3-[1-[3-[(4~{S})-6-azanyl-5-cyano-3-methyl-4-propan-2-yl-2~{H}-pyrano[2,3-c]pyrazol-4-yl]-5-(trifluoromethyl)phenyl]piperidin-4-yl]propanoic 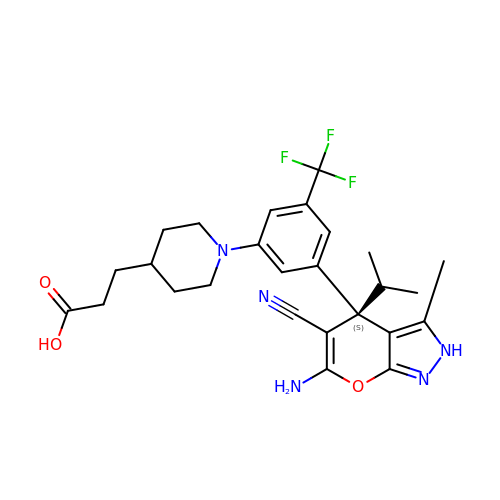acid | C26 H30 F3 N5 O3 | FJQQQYACRNHDIU-VWLOTQADSA-N> GLAEKLVPAKKVKNGVLYKSGHIKVSNVRCSYPHLDKPYGGEDGGEPKYSITLLMPKDTHGAIKKIIDEQIELTKKNHKTGALKVAPSMLFIKDGDVDFPDKPECEGMWVISARESTRPDVLNMEREELESPNEIAEEIYGGCWVSSVIRPWSQENKYGKRINANLLSVLKRKDDEPFGE

The hypothetical protein ORF6 of the Enc34 phage is conserved among all Nazgul-like phages and consists of a single domain, currently annotated as a domain of an unknown function DUF2815. Here, we present structural and functional characterization of the Enc34 ORF6 that allows us to establish its function as a single-stranded DNA-binding protein (SSB) and extend this annotation to other DUF2815 family members. The SSBs are ubiquitous within all kingdoms of life and in DNA viruses, and protect ssDNA intermediates during replication, repair and recombination. In this study, we show that the Enc34 ORF6 is structurally homologous to the gene 2.5 protein from bacteriophage T7, and present a high-resolution structure of ORF6 in complex with ssDNA, which reveals for the first time the structural basis for the ssDNA-binding mechanism of T7-type SSBs.

While co-crystallization attempts using the full-length protein were unsuccessful, the truncated ORF6ΔC protein could be crystallized both in absence of DNA and in presence of oligo-thymidine (dT). The ORF6ΔC-(dT)35 crystals diffracted to 1.56 Å and contained a single chain of ORF6ΔC in the asymmetric unit bound to a stretch of nine thymidine nucleotides. The complex structure reveals the DNA strand stretching across the entire ligand-binding surface of the OB-fold domain, which is largely positively charged and enclosed by loops L12, L23′3 and L45 that connect strands β1 and β2, β23′ and β3, and β4 and β5, respectively. The interaction thus involves portions of all five strands of the β-barrel and buries a total of 891 Å2 of the solvent-accessible surface of the ORF6ΔC protein. Upon ssDNA binding, the core of the domain remains unchanged, but the cleft-defining loops L12 and L23′3 shift to accommodate the nucleic acid and, as a result, become ordered compared to the structures without bound DNA. The protein-DNA interface reveals an extensive network of interactions that involves both stacking of aromatic side chains with DNA bases and a number of hydrogen bonds and electrostatic interactions between the protein and the DNA. The three 5′-terminal bases (T1-T3) form a slightly slanted stack, which at the 3′ end is topped by the indole ring of Trp150. The T4 base stacks with the side chain of Tyr156, resulting in a prominent twist in the DNA backbone which causes the base to face away from the protein. Following the T4-T6 stack, the bases T7 and T8 are buried in-between loops L12 and L23′3, causing another bend in the sugar-phosphate backbone. Accordingly, it is likely that the structure of ORF6ΔC-(dT)35 represents one of several possible DNA-binding states which are nevertheless similar in the underlying interactions for DNA recognition.>FCLTLRRRYTMGSSHHHHHHLEVLFQGPHMLHLVLYQPEIPQNAGNVARTAAALGWPLHLIRPLGFLLSSPKLKRAGLDYWPHVDLRLHDSFAAFLEALPRGARVFAFSARGEASLYEARFREGDYLLFGPESRGLPEEVLARFPTLKIPMPGPVRSL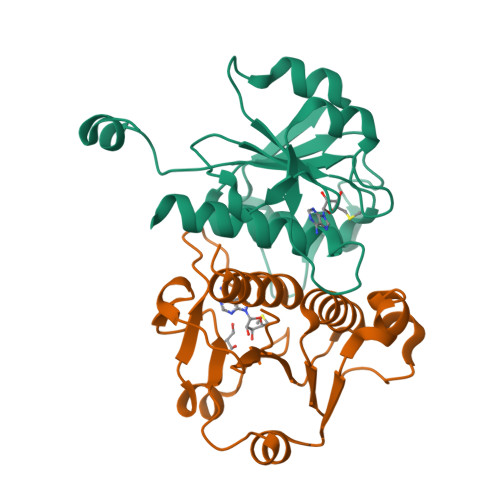NLAVAVGVAAYEAYRQLTGR[2x]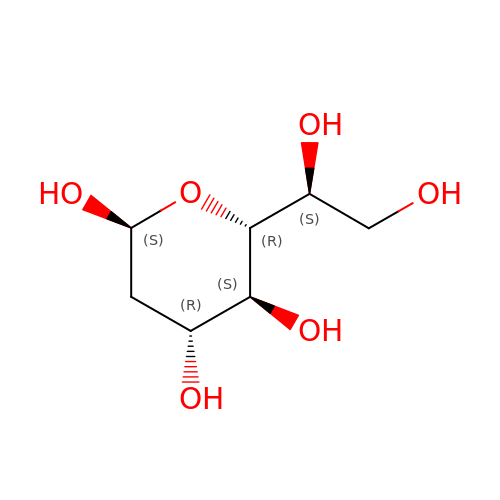2-deoxy-beta-L-galacto-heptopyranose | C7 H14 O6 | XKBYYTRLKVABMB-PFCGLBSHSA-N> IESIIKTATDTVKSEINAELGVVPSLNAVETGATSNTEPEEAIQTRTVINQHGVSETLVENFLSRAALVSKRSFEYKDHTSSAAQADKNFFKWTINTRSFVQLRRKLELFTYLRFDAEITILTTVAVNGSGNNTYVGLPDLTLQAMFVPTGALTPEKQDSFHWQSGSNASVFFKISDPPARITIPFMCINSAYSVFYDGFAGFEKNGLYGINPADTIGNLCVRIVNEHQPVGFTVTVRVYMKPKHIKAWAPRPPRTLPYMSIANANYKGKERAPNALNAIIGNRDSVKTMPHNIV;> SPSAEACGYSDRVLQLKLGNSAIVTQEAANYCCAYGEWPNYLPDHEAVAIDKPTQPETATDRFYTLKSVKWETGSTGWWWKLPDALNNIGMFGQNVQHHYLYRSGFLIHVQCNATKFHQGALLVVAIPEHQRGAHNTNTSPGFDDIMKGEEGGTFNHPYVLDDGTSLACATIFPHQWINLRTNNSATIVLPWMNAAPMDFPLRHNQWTLAIIPVVPLGTRTTSSMVPITVSIAPMCCEFNGLRHAITQ;> GVPTYLLPGSGQFLTTDDHSSAPALPCFNPTPEMHIPGQVRNMLEVVQVESMMEINNTESAVGMERLKVDISALTDVDQLLFNIPLDIQLDGPLRNTLVGNISRYYTHWSGSLEMTFMFCGSFMATGKLILCYTPPGGSCPTTRETAMLGTHIVWDFG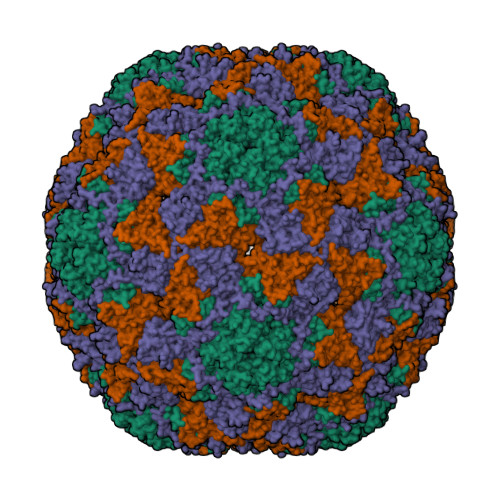LQSSVTLIIPWISGSHYRMFNNDAKSTNANVGYVTCFMQTNLIVPSESSDTCSLIGFIAAKDDFSLRLMRDSPDIGQLDHLHAAEAAYQ> MSSPCCVAIRRVARTTLESGRRQVDSKSTDVSPFFTGTQQMSLPSAGMVTKIRNFSS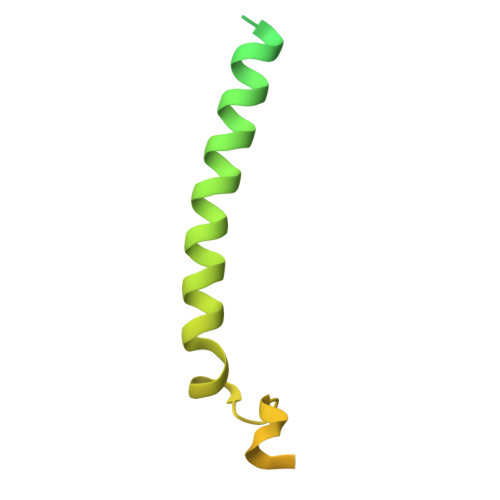VKFMDQKRSGEETVYFKKEDEALLRNLLANHPEYDPKYSVDHMNAEVGSIARDITLACQKHGMKDPSAAFMKDLISIFGAHGYAKNSK>[15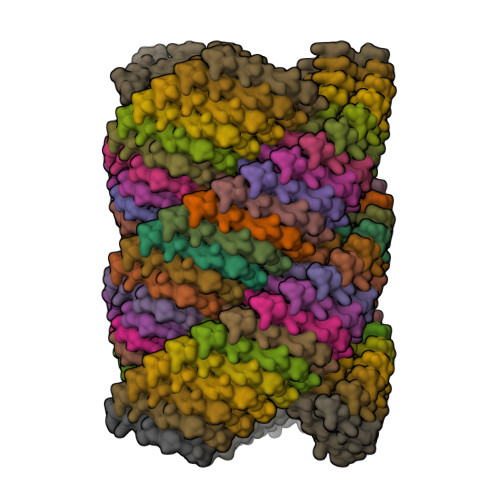0x]QAEILEADARILRAYAEILKAHAEILKAQ>[2x]MADDQ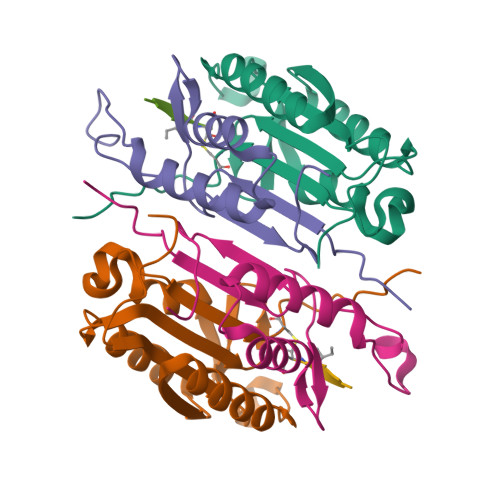GCIEEQGVEDSANEDSVDAKPDRSSFVPSLFSKKKKNVTMRSIKTTRDRVPTYQYNMNFEKLGKCIIINNKNFDKVTGMGVRNGTDKDAEALFKCFRSLGFDVIVYNDCSCAKMQDLLKKASEEDHTNAACFACILLSHGEENVIYGKDGVTPIKDLTAHFRGDRCKTLLEKPKLFFIQACRGTELDDGIQAD;>SGPINDTDANPRYKIPVEADFLFAYSTVPGYASMRNPGRGSWFVQALCSILEEHGKDLEIMQILTRVNDRVARHFESQSDDPHFHEKKQIPCVVSMLTKELYFSQLEHHHHHH[2x]>[2x]MNEQLN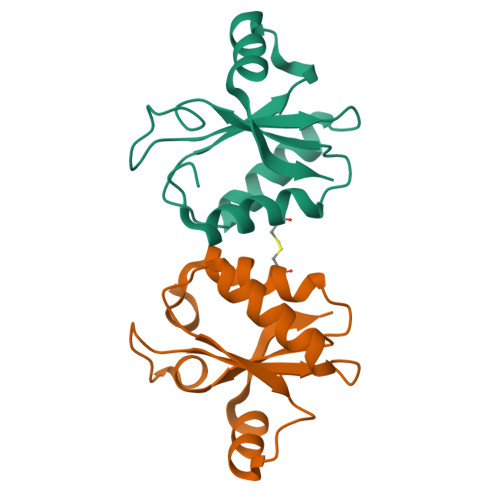HLYGLPSHAIEALKCVFKEYSQIDNAILYGSRAKGTYHQGSDIDMCLTGNLLGITELLAIENKIDDLLLPWKVDISLKHTIDNPDLLEHIERAGILFYTKES> MGAINAPAVTDDYLFSKSLAQFSSIRSGSPYADQLDWSSDGCSWSPDNPFGFKFLPACHRHDFGYRNYKRQARFNETSRLRIDDNFKSDLYHQCAGNWACNRT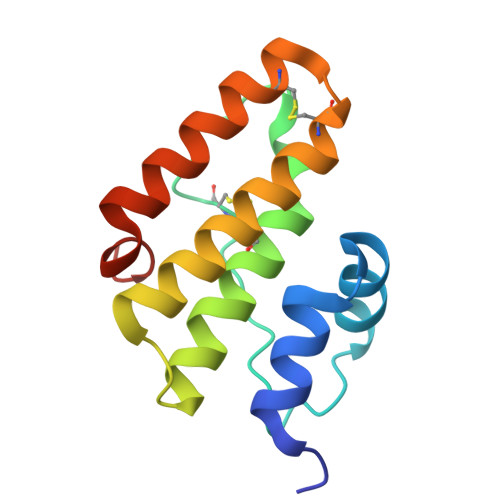ADLYYEAVRKFGASLEHHHHHH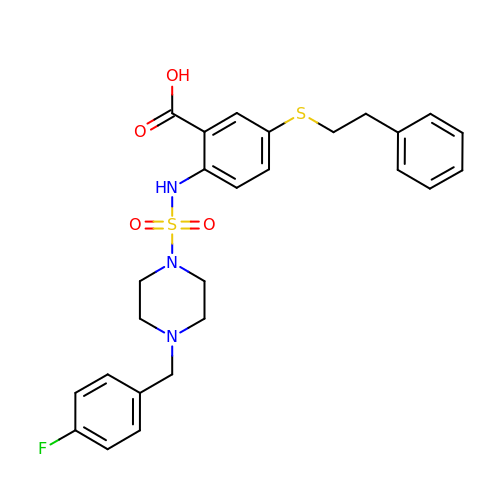2-[({4-[(4-fluorophenyl)methyl]piperazin-1-yl}sulfonyl)amino]-5-[(2-phenylethyl)sulfanyl]benzoic acid | C26 H28 F N3 O4 S2 | WLQPDKMUGJLFLQ-UHFFFAOYSA-N>[2x]GTFTGIDPFTGTQACITAASAVSGIIADLDTTIMFATAGTLNREGAETFADHREGILKTAKVLVEDTKVLVQNA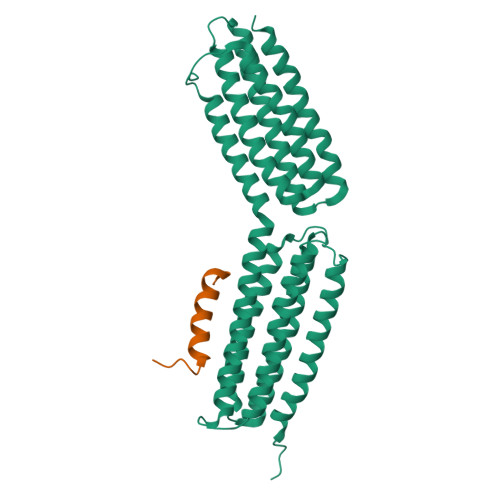AGSQEKLAQAAQSSVATITRLADVVKLGAASLGAEDPETQVVLINAVKDVAKALGDLISATKAAAGKVGDDPAVWQLKNSAKVMVTNVTSLLKTVKAVEDEATKGTRALEATTEHIRQELAVFCSPEPPAKTSTPEDFIRMTKGITMATAKAVAAGNSCRQEDVIATANLSRRAIADMLRACKEAAFHPEVAPDVRLRALHYGRECANGYLELLDHVLLTLQKPNPDLKQQLTGHSKRVAGSVTELIQAAEAMKGT;>[2x]TLDIDQSIEQLNRLILELDPTFEPIPT>MKTIIINGVQFNTDEDTTILKFARDNNIDISALCFLNNCNNDINKCEICTVEVEGTGLVTACDTLIEDGMIINTNSDAVNEKIKSRISQLLDIHEFKCGPCNRRENCEFLKLVIKYKARASKPFLPKDKTEYVDERSKSLTVDRTKCLLCGRCVNACGKNTETYAMKFLNKNGKTIIGAEDEKCFDDTNCLLCGQCIIACPVAALSEKSHMDRVKNALNAPEKHVIVAMAPSVRASIGELFNMGFGVDVTGKIYTALRQLGFDKIFDINFGADMTIMEEATELVQRIENNGPFPMFTSCCPGWVRQAENYYPELLNNLSSAKSPQQIFGTASKTYYPSISGLDPKNVFTVTVMPCTSKKFEADRPQMEKDGLRDIDAVITTRELAKMIKDAKIPFAKLEDSEADPAMGEYSGAGAIFGATGGVMEAALRSAKDFAENAELEDIEYKQVRGLNGIKEAEVEINNNKYNVAVINGASNLFKFMKSGMINEKQYHFIEVMACHGGCVNGGGQPHVNPKDLEKVDIKKVRAS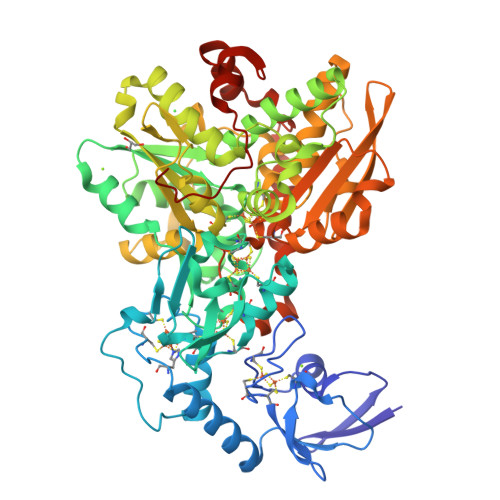VLYNQDEHLSKRKSHENTALVKMYQNYFGKPGEGRAHEILHFKYKKSAWSHPQFK[2x]>MYVYKRDGRKEPVQFDKITARISRLCYGLDPKHIDAVKVTQRIISGVYEGVTTIELDNLAAETCAYMTTVHPDYATLAARIAISNLHKQTTKQFSKVVEDLYRYVNAATGKPAPMISDDVYNIVMENKDKLNSAIVYDRDFQYSYFGFKTLERSYLLRINGQVAERPQHLIMRVALGIHGRDIEAALETYNLMSLKYFTHASPTLFNAGTPKPQMSSCFLVAMKEDSIEGIYDTLKECALISKTAGGIGLHIHNIRSTGSYIAGTNGTSNGLIPMIRVFNNTARYVDQGGNKRPGAFALYLEPWHADIFDFIDIRKN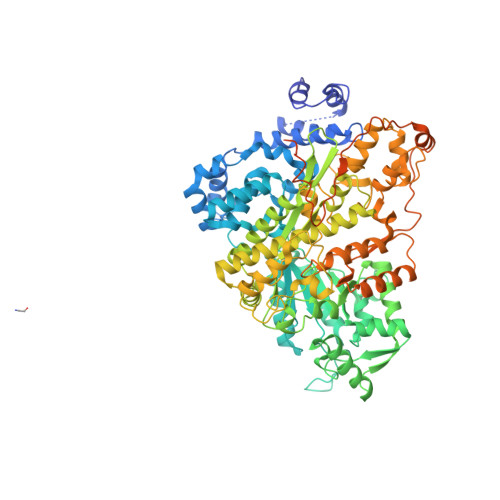HGKEEIRARDLFPALWIPDLFMKRVEENGTWTLFSPTSAPGLSDCYGDEFEALYTRYEKEGRGKTIKAQKLWYSILEAQTETGTPFVVYKDACNRKSNQKNLGVIKSSNLCCEIVEYSAPDETAVCNLASVALPAFIETSEDGKTSTYNFKKLHEIAKVVTRNLNRVIDRNYYPVEEARKSNMRHRPIALGVQGLADTFMLLRLPFDSEEARLLNIQIFETIYHASMEASCELAQKDGPYETFQGSPASQGILQFDMWDQKPYGMWDWDTLRKDIMKHGVRNSLTMAPMPTASTSQILGYNECFEPVTSNMYSRRVLSGEFQVVNPYLLRDLVDLGIWDEGMKQYLITQNGSIQGLPNVPQELKDLYKTVWEISQKTIINMAADRSVYIDQSHSLNLFLRAPTMGKLTSMHFYGWKKGLKTGMYYLRTQAASAAIQFTIDQKIADQATENVADISNLKRPSYMPSSASYAASDFVPAAVTANATIPSLDSSSEASREASPAPTGSHSLTKGMAELNVQESKVEVPEVPAPTKNEEKAAPIVDDEETEFDIYNSKVIACAIDNPEACEMCSG[2x]Type III CRISPR systems are innate immune systems found in bacteria and archaea, which produce cyclic oligoadenylate (cOA) second messengers in response to viral infections. In these systems, Csm6 proteins serve as ancillary nucleases that degrade single-stranded RNA (ssRNA) upon activation by cOA. In addition, Csm6 proteins also possess cOA-degrading activity as an intrinsic off-switch to avoid degradation of host RNA and DNA that would eventually lead to cell dormancy or cell death. The two TtCsm6 monomers dimerize in an X-shape, and each monomer contains an N-terminal CARF domain, an intermediate helix-turn-helix (HTH) domain and a C-terminal HEPN domain.

The T59A or S60A single mutation did not have a significant effect, but the T59A/S60A double mutation and K137A single mutation abrogated cA4 cleavage, consistent with their conserved roles in cA4 cleavage. In addition, T81A was about 100-fold weaker, and K137A completely lost its ability to bind cA4, suggesting that these residues mainly contribute to cA4 binding. In contrast, mutation of T59A/S60A or K137A completely eliminated RNA degradation activity. In the previously reported structure of apo-TtCsm6, residues N416 and H422 are coordinated by a Ni2+ ion, which may cause a conformational distortion and hence generate an artifact. Coincidentally, in the structure of TtCsm6K137A, which we initially determined to investigate the impact of K137A mutation on the structural integrity of TtCsm6 homodimer, no metal ions were detected in the HEPN domain. The Ni-free structure of TtCsm6 is essentially identical to that of the Ni-bound one both in the overall structure and in the R-X4-6-H motif. Thus, Ni2+ ion-binding does not significantly change the active site arrangement of HEPN domain. In the apo state, N416 and H422 of monomer-1 form hydrogen bonds with H422’ and N416’ of monomer-2, respectively, and the guanidine group of R415 is buried inside the domain, where it is stabilized by E332.

>[2x]SGRPMEDLDALWERYREAVRAGGNPQALYQEMVWPALLALWREKPRVYPFPQAFAVSVHTLGTSPEATALAILGAGAERVYVLHTPESARFLPRLRQDTGKDLYPVEIGKSDVEAIYREVKRLLEKHPEVPVALDLTSGTAAMSAGLAAAGFFFQRFYPKVRVVYVDNEDYDPELRRPRAGTEKLRILPNPHEALAEVDALFAKELYGKGEFGQAAAYFRGMVGRTGNQAYALYALLAEMYRAWRALDFGEALKAGRKLLGQLSQNVWLNHPLNARREALEAQVALLEAVDRFLKARDFALKEGVYGLARTLLHLAQEAKEEAAVLAALYAYRALELLLQERLALLGRRAEAPGLSPEEAEALRKALAELLGVLPEEVRLPAKLGLLDLLAFLRLKGDEALGRLSLAELRGLAGALKGRNSALLVHGFDVPSPKAVEGIARLAQGLLQDLEARTALGPLSPEPVPLGF> MSENFKWNLGNNLNSNNNDDFFSTQPFNNNNKFDFSILPDDNNEDEFSGIVNNNNNMNNNNTLVKGDGGIFGNTQINFNNNNNNNNQFGNSLFGNTINNNNNNMEVNNDNDNNNNEQEFEMDNQQLQNNQMEMEEDENQFNNIFNDKSRTDDTIYHNTLEYELQPKLNDDPHLIPIELSDTFLKLSQAKINSINDDESNKLFYMQNNRKQKEQQLKNYQMEKDTWSILKKLYEYRDIQRSIDQKEKIDISQPNQVQVYNYLIKKDHKLRENLILLEWLEEMSSQVELNDNDAVFWEYTLIKLKKSNSITMLTNNQMVSELDPDAMSRQNKPIDKDDEKNQSRFLKTVWSFLRAGDRVGAAEYCTNVGQFWRAQTLIGLNYYQGEHSIGNPYFNLWKSNCLNISKNSNDQYERAIYGLLCGNLEATLPIQKNWYDYFWCYLRVLYDESLYRELKPYRSPLSIEEDIDSPPSTCISQINTPKDILEILKNNTSQIEIKNQSENPYHQIQELIIADDYSILFNSLPNLLLKNKTPEFNRFAVLLIL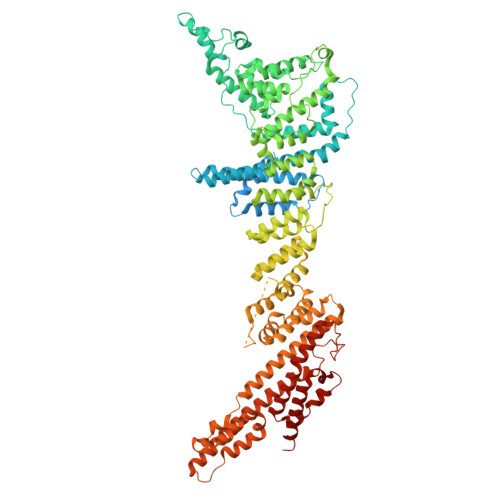FFRKREQYELISTSEDCPENIVINEYVQHLINSQQYELVALYTSLLNNESLQVDVYSRFLVNIIDPNQRQQLLVLAEKFGLNTQEIAQSVVKTITSGSINTTSNSFENLEFTGFATTINKNKQPKNKSTTTTKASTTETTTNTNTTTTPNLTNTIINQDSSITTQDDLVKINSIQWLCFEKQLLIKAILQSNLLLRDFISLNKYGAASELLKSLPKDIVMIAKQQSPLNESDTNNIIKEFRDWENYITANIRINLWLQNYSNQPKISNYLPQSLNNNNNYINNNNNSFNNIINNSIINSSIAFRLRGNESYAEKLDIERRKKEYDDVYGQWNQNNINFGKEAIVSIRSIIKTGWLCPLENQIGLFSEDDQSGHEVTLIRKKCIPSLFKSLYTILVGIGSIQKSSQLCNQIANERFRWYSIFSKKELQEILQLVRESSIKLLN> GTIARTIVLQESIGKGRFGEVWRGKWRGEEVAVKIFSSREERSWFREAEIYQTVMLRHENILGFIAADNKDNGTWTQLWLVSDYHEHGSLFDYLNRYTVTVEGMIKLALSTASGLAHLHMEIVGTQGKPAIAHRDLKSKNILVKKNGTCCIADLGLAVRHDSATDTIDIAPNHRVGTKRYMAPEVLDDSINMKHFESFKRADIYAMGLVFWEIARRCSIGGIHEDYQLPYYDLVPSDPSVEEMRKVVCEQKLRPNIP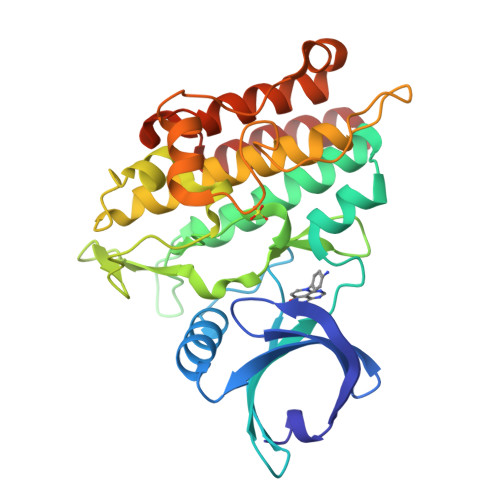NRWQSCEALRVMAKIMRECWYANGAARLTALRIKKTLSQLSQQEGIKM Arginine kinase (AK) plays a crucial role in the survival of Daphnia magna, a water flea and a common planktonic invertebrate sensitive to water pollution, owing to the production of bioenergy. AK belongs to the phosphagen kinase family and acts as an energy modulator when bioenergy is required in invertebrate cells, by reversibly converting phosphoarginine and ADP to L-arginine and ATP. In structural aspects, both AKapo and AKholo have been shown to consist of two domains, an arginine interacting in the N-terminal domain and ATP in the C-terminal domain. AK from D. magna (DmAK) has four highly conserved histidine residues, namely, H90, H227, H284, and H315 in the amino acid sequence.

In this study, we report for the first time the crystal structure and stability of the D. magna arginine kinase (DmAK) H227A mutant, which is close to the L-arginine binding site. In the final refinement at 1.75 Å, Rwork and Rfree values of DmAK H227A were 0.181 and 0.224, respectively. The overall structure of DmAK H227A had 360 amino acids, 320 water molecules, and 1 ion each of PO43− and NO3−. Although cocrystallization with ADP and L-arginine substrates was conducted, their presence was not detected in the DmAK H227A structure. The root-mean-square deviation was estimated as 0.326 Å for Cα atoms in the superposition of DmAK WT and H227A. In the case of the DmAK H227A structure, the hydrogen bond destruction between A135 and H227, resulted in the replacement of one water molecule (WAT684) at the imidazole group of histidine position. Moreover, the disruption of the hydrogen bond decreased the stability of the secondary structure of DmAK H227A. In the crystal structure of DmAK H227A, the hydrogen bond disruption between H227 and A135 resulted in the lowered structural stability of DmAK H227A due to the weakness of α-helix formation of the FNPCL residues as also shown by CD signal data. In the enzyme kinetics and stability assay, the H227A mutant revealed a 18% lower activity and an extremely lower structural stability than the WT. The highly conserved H227 residue adjacent to the arginine binding site affected the structural stability of DmAK, and the turnover (Kcat) value of H227A decreased by about 17.9% compared to the wild type as shown by the enzyme kinetic results.

> HHHHMVDAAVAEKLEAGFQKLQEATNCKSLLKKHLTREIFDKIKDLKTSFGSTLLDVIQSGVENLDSGFGVYAPDAEAYSVFNDLFEPMICDYHTGFKPGDAHPPRDFGDLETFGNLDPEGAFIVSTRVRCGRSLAGYAFNPCLTEANYKEMEEKVVASLSSLEGELKGTYYPLTGMTKEVQTQLIQDRFLFKEGDRFLQAANACRYWPTGRGIYHNDAKTFLVWCNEEDALRIISMQKGGDLKAVYARLVNAINEIEKRIPFSHHDKYGFLTFCPTNLGTTIRASVHIALPKLAADLAKLEEAAGKFNLQVRGTAGEHTEAEGGVYDISNKRRMGLTEYQAVKEMYDGLQELIRMEKEA2-(3,4-dimethoxyphenyl)-5-(piperidin-4-yl)-3-(propan-2-yl)-1H-indole 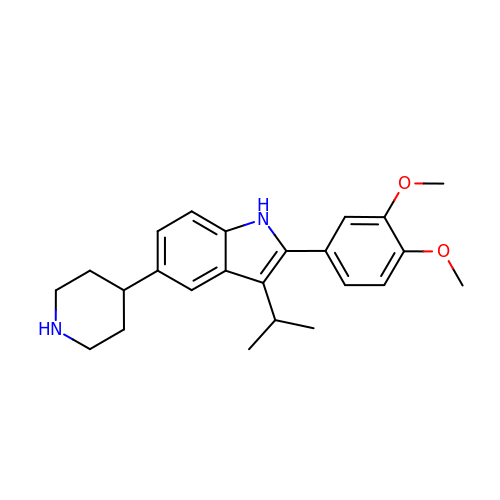| C24 H30 N2 O2 | XKWJVTCJPRLPJR-UHFFFAOYSA-N>GRDKDHLLKYNVGDLVWSKVSGYPWWPCMVSADPLLHSYTKLKGQKKSAR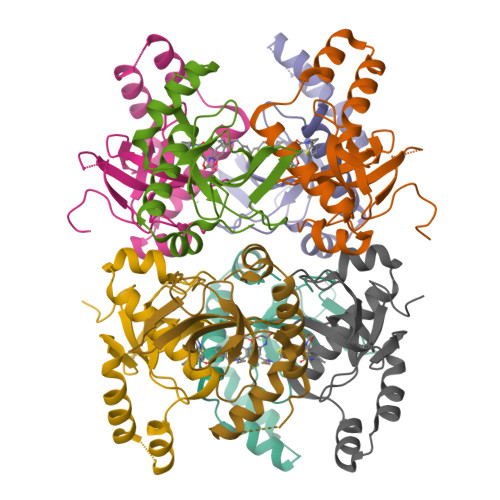QYHVQFFGDAPERAWIFEKSLVAFEGEGQFEKLCQESAKQAPTKAEKIKLLKPISGKLRAQWEMGIVQAEEAASMSVEERKAKFTFLYVG[8x]> VVGGTEAQRNSWPSQISLQYRSGSSWAHTCGGTLIRQNWVMTAAHCVDRELTFRVVVGEHNLNQNNGTEQYVGVQKIVVHPYWNTDDVAAGYDIALLRLAQSVTLNSYVQLGVLPRAGTILANNSPCYITG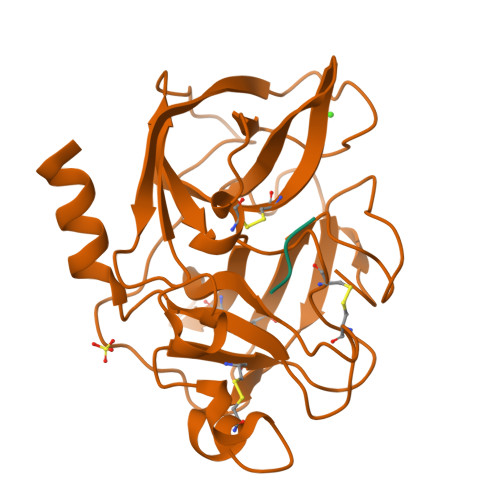WGLTRTNGQLAQTLQQAYLPTVDYAICSSSSYWGSTVKNSMVCAGGDGVRSGCQGDSGGPLHCLVNGQYAVHGVTSFVSRLGCNVTRKPTVFTRVSAYISWINNVIASN;> YPFVEPIDF>GPAMAKVETGTDVTSKVTVEIGSIEGHNNTNKVEPHAGQRAVLKYKLKFENGLHQGDYFDFTLSNNVNTHGVSTARKVPEIKNGSVVMATGEVLEGGKIRYTFTNDIEDKVDVTAELEINLFIDPKTVQTNGNQTITSTLNEEQTSKELDVKYKDGIGNYYANLNGSIETFNKANNRFSHVAFIKPNNGKTTSVTVTGTLMKGSNQNGNQPKVRIFEYLGNNEDIAKSVYANTTDTSKFKEVTSNMSGNLNLQNNGSYSLNI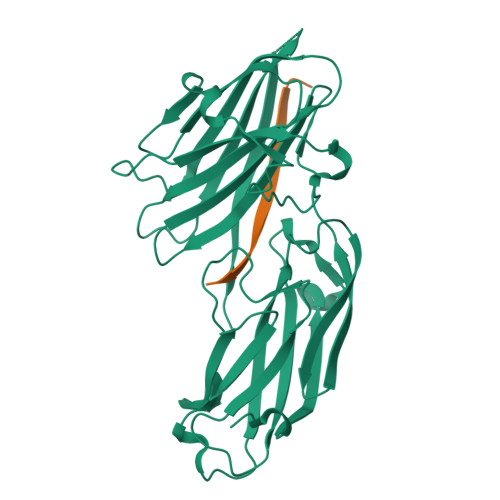ENLDKTYVVHYDGEYLNGTDEVDFRTQMVGHPEQLYKYYYDRGYTLTWDNGLVLYSNKA[2x];>GEGQQHHLGGAKQAGDV[2x]>GHMAEPRIVVLGAGPAGAATAIGLRRLGYAVTVVSEWRRFAAVEGVSQRVLEGLRHVGLGGALRQAAMPATRQVHWNGQQLHLNQEFLLDRQRFDRALRDDLQRAGVSVVEGRVREVVRDVGHGIRLDDGQVLQADFLVEARGRQAPLAADRLRGPETVSLLNVWQAAPGAPASAVESLADGWAWMARLEDGRCYWQVTLDAAGLPGKAGLADYCAARRADSALVTELFDARALASAEVHARSSTAILAGECVGQDWIRVGDAAMAVDPLSGNGIFQSLSSALQAPVVINTLLRRPERAGLARQFHQQRIEQLFLRFARIGRDFYGQEQGRVGQPFWARRQGWPDMQALHVAADWSAVRVERRPVL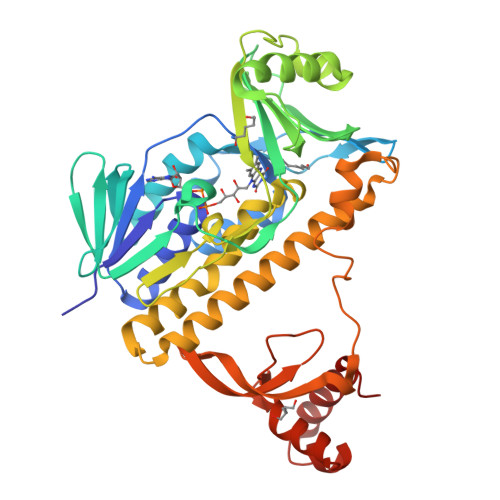RDGLVDEAEVVVTADQPLGVWHLQGVELAPAVRELQAGRPLEAVVSGLSGEQQRMVRRWLLEQGLV[2x]>[2x]MYKIIGREIYGKGRKGRYIVKFTRHWPQYAKNIYLIGEFTSLYPGFVKLRKIEEQGIVYLKLWPGEYGYGFQIDNDFENVLDPDNEEKKCVHTSFFPEYKKCLSKLVIKEPDNPLDKIIHIEESGFIHKFNGEIIIRLIAPTEINEPLIDLGNEIREPLTKHVVGDNIVYQYIIPSRSILRYRFIFNYNDKKLFYGDEGVSENSSYIVVNSKYIPGVDKPRWYMGTVYYQIFIDSFDNGDPNNDPPNRIKKTVPREYGYYGGDLAGIMKHIDHLEDLGVETIYLTPIFSSTSYHRYDTIDYKSIDKYLGTMEDFEKLVQVLHSRKIKIVLDITMHHTNPCNELFVKALREGENSPYWEMFSFLSPPPKEIVELMLKYIDGEECRSRELYKLDYFRNNKPFYEAFFNIWLMAKFNHDNPR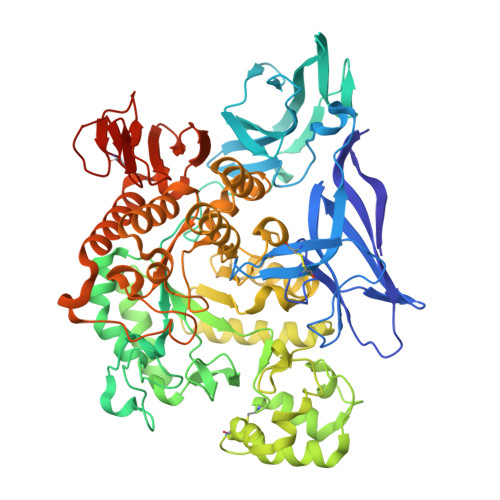TVDYFIDITKFWIDKGIDGFRIDVAMGIHYSWMKQYYEYIKNTYPDFLVLGELAENPRIYMDYFDSAMNYYLRKAILELLIYKRIDLNEFISRINNVYAYIPHYKALSLYNMLGSHDVPRIKSMVQNNKLLKLMYVLIFALPGSPVIYYGDEIGLEGGRDPDNRRPMIWDRGNWDLELYEHIKKLIRIYKSCRSMRHGYFLVENLGSNLLFIKRWINNEEIIFLLNVSSKDISVDLKKLGKYSFDIYNEKNIDQHVENNVLLRGYGFLILGSKPCNI>[2x]GMQNPVATVLLLQGDLYCSPNCLATFQDQARRDSFGIQSKVALKTFAAADQREAEGRDLRTAYNEIATDIGRSQQINENIIKYPPGNHVLSGGLMTPFHALAHGMFGLGAPLTFPIQNV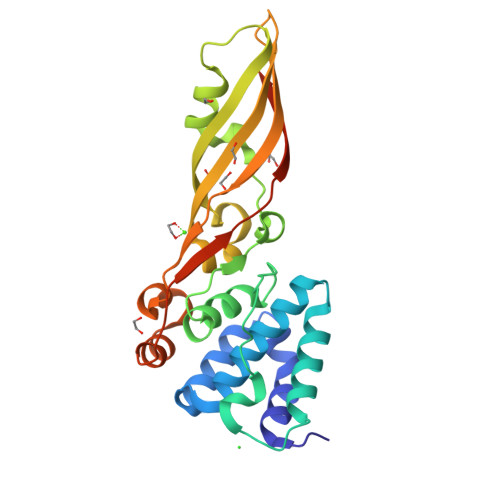GLNVDIRGIPDVMNVIQSARPVGTSSLDVNFAYDVGKDSNASWLTLGNITLRLVGTIDKNASGAWTFSGEIRAFNDVYDANPSNHRGWLGENLTSLLSAVPFTSYSIEIPGSLPVTVSGNLEHHHHHH N. maritimus, like most archaeal cells, is encased by a paracrystalline, proteinaceous surface layer or S-layer. The structure shows that the S-layer is pseudohexagonal and consists of the repeated interactions of the Nmar_1547 (hereafter, NmSLP) S-layer protein. At the sequence level, NmSLP is arranged into ten immunoglobulin-like (Ig-like) domains. Collectively, our structural data reveal that the S-layer of N. maritimus functions as a multichannel exchanger for ammonium ions, featuring negatively charged residues that line several pores in the S-layer.

Our goal was to solve the structure of the N. maritimus S-layer directly from whole cells. Using subtomogram averaging, we mapped the locations of the S-layer repeating units on the cell, which were arranged in a hexagonal array. As a result, we produced a high-resolution map of the N. maritimus S-layer hexamer from intact cells. The central region of the S-layer hexamer in the map had a resolution of 3.3 Å, with the resolution decaying to around 4.5 Å towards the periphery. The first eight domains were well resolved in our 3.3–4.5-Å-resolution subtomogram averaging map. By contrast, the last two domains appeared less ordered, with the local resolution decaying towards the C terminus of NmSLP, away from the centre of the S-layer hexamer. Each monomer of NmSLP in the S-layer adopts a rough ‘cashew’ shape, facilitating several interactions around the hexamer of NmSLP. Domain 4, nestled within domain 3 and linked by short connectors, is slightly raised relative to the base of the cashew-shaped Ig-array of NmSLP, projecting towards the extracellular milieu.

>[6x]MNNEIGRKITSLTLMTIMVAGGLTFAIPGVMPEAMAANANLFVSAENSQFDNYMSGPQVIEVVVIDSDINDTDEAKGEPDVTVNGKVLRMVQAVDGNWYGYFADRDQAQIADSTATTADSGLDFGVFCASSSGTAALGFSTTETDGIAIPITIANATATGNGTQTGSSSGGAITTTCAANTLDASTANGTINVVREAKDPVAASGSVSVGQIGLKNGTANSGPNWPFIQLYELNPTGNVVVQYNKGGGVQSTTLTFDTVDQFAELSLDRTVFPRVSQVHATITDLWLNIDPTDEDSWTFATNTKNTTSSFNVDTFYQVFDENGASGGSALTLRTTLSSLMCEDNCVLTLDVDAQSSGTPVVTIQDNGDSILTQLNASSNTNANNASAFGISTETAKLGTGSIPVTITEQGPNSGVFGTYDESDKSVLKITDNAKRGTSASLDYNETPQTILVGFSFASIDIQPVTDEWTSGQEIPVVIVDADQNKNSRADEDLDLNNPDVTLIPALRTGDPFTIDEGGTPSLIFTNGTNGDDSIFDTGAINNTSAGQVGNFTLNINVTRFSSATNITSTESIDTFSKRLISAQTANSSANFDVDFAIIDLGSATLETLKETVVDEDNTAVGFNFFNYDVRSLGADTVSIALLNTTGNILPWVNNDTRNVDKNNAILLVSNSTNSQAYVDLTNAVSDAVYGSTNTDSNVNIGFAMYFTGVGDLAAKEVIVMDFFSFGFTDDGVQSSERFANQIIRIEAEETGDNTSTFEGSLEYVMVNQINIQDAGTFSGITPIADDPSFIVIEDLTDEDAPRVNYNDLGADGVTTPVSDQEEAPSHSGVVSLNADSYKIADTVVITVEDLDLNVDSDLIDIFTVVSDNSKATDDAVGSATTQSLSFGELGRLLDVTFDDVIWSTPDGANNTATGNDSDTCSTELSNAGITDTGLGATGFTLVETGAATGVFVGDFQIPSFWCRVSDTTTTPYTYAGDEETTTGLDIEVNYVDFRDASGEIVEVGDSAGVRANTGSVSLDRTVYPVPFGTIADSSKAANAAPNGRSVFPIHATGITSTIDSTEELPTGDLTIHVRINDPDFDENPAGEDAMDQDNALKISVIRGSDSVVLGYAGASERTGKIDVGGNNGTISNIRSFGEMDEIAPDAGIFELDVNIKFTDGPASAQCNSHDTLYTALDGTTGKADTNRFDDGAASGQEYCILQGDILQVEYTDPADASGDANTVTDSATFDLRNGVLQSDKSVYIIGSDMILTLIEPDFDLDNDSAETYDLDLIEWDSDAATTTMGNKGVTGAAAAFDPEPTDFRETGDSTGIFQIVIEIPESLSNDKLERGEEIILEYTDWGPSGSDYVGDEDEDVNLTIYTSNFGATVELDQKVYSWTDKVYITIVAPDHNFDSDLVDEIGETDSDPIKVSTRGFDLDNYKLVETGTDTGIFTGEVILTGFTAHDADGDGNTGDATGTTSGSGPTDGLLATDDDDGLTVSFEFSEDETIVGSALIRWNIGEVQWLEASYPASGTGVVRVIDPDMNLDPEAVDNFEVDVWSDSDAGGIDLTVTETNEATGIFEGTVFFTTLDESSGHRLRVSEGDTVTAEYEDNTLPDPYTTADELDITATSLIGTVVPPLERAPAANLRTVDAFGNSLDSVSVDQQVQISADLANGQDREQSFAYLVQIQDANGVTVSLAWITGSLSSGQSFSPALSWIPTEAGTYTATAFVWESVDNPTALSPPVSTTVNVS>[2x]MAREFSLEKTRNIGIMAHIDAGKTTTTERILYYTGRIHKIGETHEGASQMDWMEQEQDRGITITSAATTAA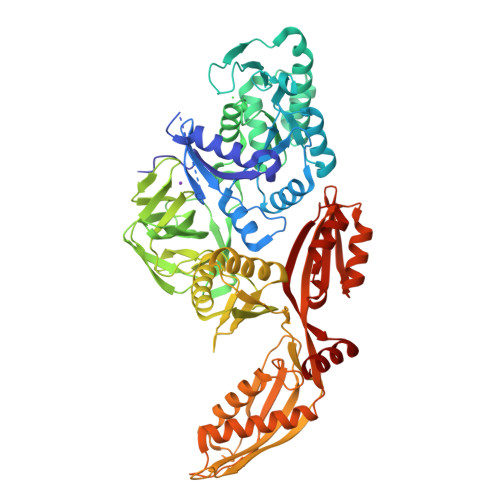WEGHRVNIIDTPGHVDFTVEVERSLRVLDGAVTVLDAQSGVEPQTETVWRQATTYGVPRIVFVNKMDKLGANFEYSVSTLHDRLQANAAPIQLPIGAEDEFEAIIDLVEMKCFKYTNDLGTEIEEIEIPEDHLDRAEEARASLIEAVAETSDELMEKYLGDEEISVSELKEAIRQATTNVEFYPVLCGTAFKNKGVQLMLDAVIDYLPSPLDVKPIIGHRASNPEEEVIAKADDSAEFAALAFKVMTDPYVGKLTFFRVYSGTMTSGSYVKNSTKGKRERVGRLLQMHANSRQEIDTVYSGDIAAAVGLKDTGTGDTLCGEKNDIILESMEFPEPVIHLSVEPKSKADQDKMTQALVKLQEEDPTFHAHTDEETGQVIIGGMGELHLDILVDRMKKEFNVECNVGAPMVSYRETFKSSAQVQGKFSRQSGGRGQYGDVHIEFTPNETGAGFEFENAIVGGVVPREYIPSVEAGLKDAMENGVLAGYPLIDVKAKLYDGSYHDVDSSEMAFKIAASLALKEAAKKCDPVILEPMMKVTIEMPEEYMGDIMGDVTSRRGRVDGMEPRGNAQVVNAYVPLSEMFGYATSLRSNTQGRGTYTMYFDHYAEVPKSIAEDIIKKNKGE>[3x]MRKFNSHSIPIRLNLLFSIVILLFMTIIGRLLYMQVLNKDFYEKKLASASQTKVTTSSARGEIYDASGKPLVENTLKQVVSFTRSNKMTATDLKEIAKKLLTYVSISSPNLTERQLADYYLADPEIYKKTVEALPSEKRLDSDGNRLSESELYNNAVDSVPTSQLNYTEDEKKEIYLFSQLNAVGNFATGTIATDPLNDSQVAVIASISKEMPGISISTSWDRKILETSLSSIVGSVSSEKAGLPAEEAESYLKKGYSLNDRVGTSYLEKQYEEVLQGKRPVKEIHLDKHGDMESVENIEEGSKGKNIKLTIDLAFQDSVDALLKSYFNSELGNGGAKYSEGVYAVALNPQTGAVLSMSGLKHDLKTGELTPDSLGTVTNV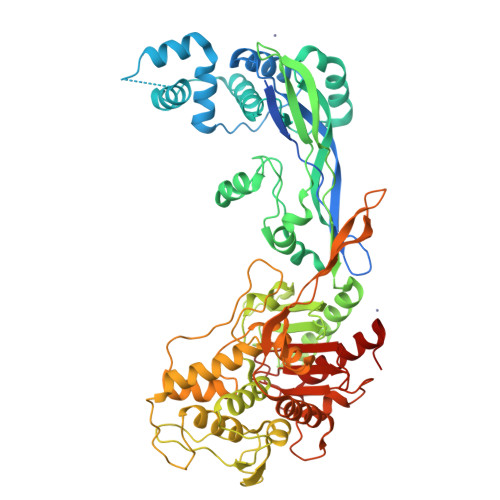FVPGSVVKAATISSGWENGVLSGNQTLTDQPIVFQGSAPIYSWYKLAYGSFPITAVEALEYSSNAYVVQTALGIMGQTYQPNMFVGTSNLESAMGKLRSTFGEYGLGSATGIDLPDESTGLVPKEYNFANFITNAFGQFDNYTPMQLAQYVATIANNGVRLAPHIVEGIYDNNDKGGLGELIQAIDTKEINKVNISESDMAILHQGFYQVSHGTSPLTTGRAFSDGATVSISGKTGTGESYVAGGQEATNTNAVAYAPTENPQIAVAVVFPHNTNLTKNVGPAIARDIINLYNQHHPMN> ADPGAPTPVNPCCYYPCQHQGICVRFGLDRYQCDCTRTGYSGPNCTIPGLWTWLRNSLRPSPSFTHFLLTHGRWFWEFVNATFIREMLMRLVLTVRSNLIPSPPTYNSAHDYISWESFSNVSYYTRILPSVPKDCPTPMGTKGKKQLPDAQLLARRFLLRRKFIPDPQGTNLMFAFFAQHFTHQFFKTSGKMGPGFTKALGHGVDLGHIYGDNLERQYQLRLFKDGKLKYQVLDGEMYPPSVEEAPVLMHYPRGIPPQSQMAVGQEVFGLLPGLMLYATLWLREHNRVCDLLKAEHPTWGDEQLFQTTRLILIGETIKIVIEEYVQQLSGYFLQLKFDPELLFGVQFQYRNRIAMEFNHLYHWHPLMPDSFKVGSQEYSYEQFLFNTSMLVDYGVEALVDAFSRQIAGRIGGGRNMDHHILHVAVDVIRESREMRL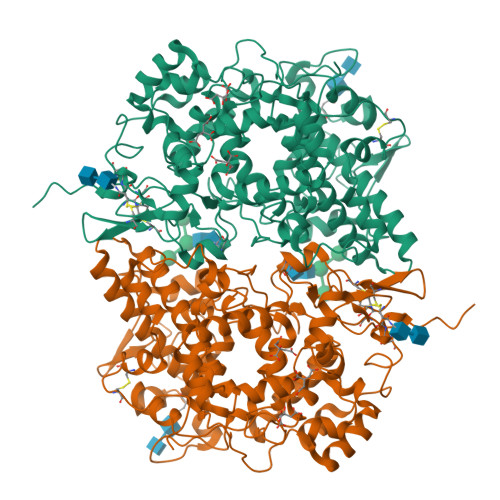QPFNEYRKRFGMKPYTSFQELVGEKEMAAELEELYGDIDALEFYPGLLLEKCHPNSIFGESMIEIGAPFSLKGLLGNPICSPEYWKPSTFGGEVGFNIVKTATLKKLVCLNTKTCPYVSFRVPDASQDDGPAVERPSTEL AsfvLIG catalyzes the DNA ligation reaction during the base excision repair (BER) process of ASFV genome. AsfvLIG is composed of 419 amino acids and is one of the smallest DNA ligases identified to date. However, unlike the homologous proteins (such as HsLIG1 and SusLIG1), the fidelity of AsfvLIG is very low. By solving four AsfvLIG:DNA complex structures, including the non-catalytic open form and the catalytic closed forms, we showed that the NTD, AD, and OB domains of AsfvLIG undergo a large conformational change during the catalytic assembly.

Among the three catalytic structures, AsfvLIG:CT2 captured one sealed C:T pair, whereas AsfvLIG:CG and AsfvLIG:CT1 captured unsealed C:G and C:T pairs at the catalytic sites, respectively. The structures belong to two different space groups: P212121 for AsfvLIG:CT2 and P21 for both AsfvLIG:CG and AsfvLIG:CT1. The molecular packing of AsfvLIG:CT2 is very different from the other two structures in the crystal lattice. However, as indicated by the low root mean square deviation values (rmsd, about 0.75 Å based on the superposition of 404 pairs of Cα atoms) among them, the three complex structures are very similar to each other. In the AsfvLIG:CT2 structure, the template C11 and the sealed T12 form one H-bond (2.9 Å) between their nucleobases. However, though the pairing and overall shape of C11:T12 pairs are similar in the AsfvLIG:CT1 and AsfvLIG:CT2 structures, superposition reveals some subtle conformational changes at the local regions. Compared to the AsfvLIG:CT1 structure, the C11-T12 pair is shifted about 0.5 Å toward the main chain N atom of Gln403 in the AsfvLIG:CT2 structure, which may exclude the C11-interacting water molecule. Meanwhile, the side chain of Gln403 rotates clock wise around the CG-CD bond for about 15° in the AsfvLIG:CT2 structure, leading to the formation of one H-bond (2.9 Å) between the NE2 atom of Gln403 and the O2 atom of the T12 nucleobase, thereby shifting the conformation to the ligated product.

>MLNQFPGQYSNNIFCFPPIESETKSGKKASWIICVQVVQHNTIIPITDEMFSTDVKDAVAEIFTKFFVEEGAVRISKMTRVTEGKNLGKKNATTVVHQAFKDALSKYNRHARQKRGAHTNRGMIPPMLVKYFNIIPKTFFEEETDPIVQRKRNGVRAVACQQGDGCILLYSRTEKEFLGLDNIKKELKQLYLFIDVRVYLDGELYLHRKPLQWIAGQANAKTDSSELHFYVFDCFWSDQLQMPSNKRQQLLTNIFKQKEDLTFIHQVENFSVKNVDEALRLKAQFIKEGYEGAIVRNANGPYEPGYNNYHSAHLAKLKPLLDAEFILVDYTQGKKGKDLGAILWVCELPNKKRFVVTPKHLTYADRYALFQKLTPALFKKHLYGKELTVEYAELSPKTGIPLQARAVGFREPINVLEII[2x]>[21x]FTLIELMIVIAIVGILAAVALPAYQDYTARAQVSEAILLAEGQKSAVTEYYLNHGKWPENNT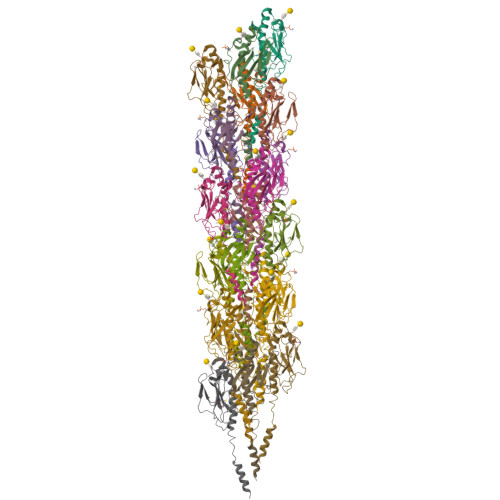SAGVASSPTDIKGKYVKEVEVKNGVVTATMLSSGVNNEIKGKKLSLWARRENGSVKWFCGQPVTRTDDDTVADAKDGKEIDTKHLPSTCRDNFDAK> GAMAMANIAVQRIKREFKEVLKSEETSKNQIKVDLVDENFTELRGEIAGPPDTPYEGGRYQLEIKIPETYPFNPPKVRFITKIWHPNISSVTGAICLDILKDQWAAAMTLRTVLLSLQALLAAAEPDDPQDAVVANQYKQNPEMFKQTARLWAH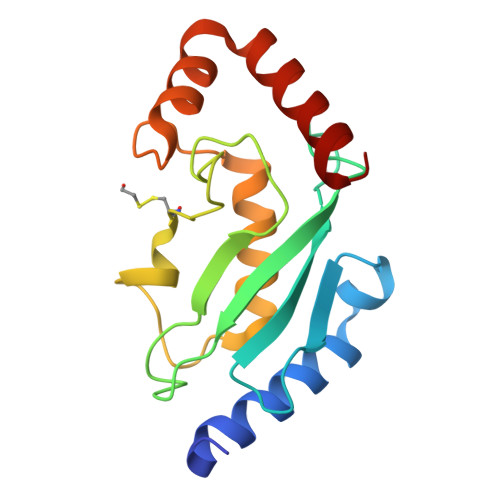VYAGA> ALTQSVGGDSSADRLFPPQWICCDIRYLDVSILGKFAVVMADPPWDIHMELPYGTLTDDEMRRLNIPVLQDDGFLFLWVTGRAMELGRECLNLWGYERVDEIIWVKTNQLQRIIRTGRTGHWLNHGKEHCLVGVKGNPQGFNQGLDCDVIVAEVRSTSHKPDEIYGMIERLSPGTRKIELFGRPHNVQPNWITLGNQLDGIHLLDPDVVARFKQRYPDGIISKPKNL;> LKGTQSLNPHNDYCQHFVDTGHRPQNFIRDVGLADRFEEYPKLRELIRLKDELIAKSNTPPMYLQADIEAFDIRELTPKFDVILLEPPLEEYYRETGITANEKCWTWDDIMKLEIDEIAAPRSFIFLWCGSGEGLDLGRVCLRKWGYRRCEDICWIKTNKNNPGKTKTLDPKAVFQRTKEHCLMGIKGTVKRSTDGDFIHANVDIDLIITEEPEIGNIEKPVEIFHIIEHFCLGRRRLHLFGRDSTIRPGWLTVGPTLTNSNYNAETYASYFSAPNSYLTGCTEEIERL

The m6A RNA modification is catalyzed in the nucleus by a multiprotein writer complex containing the putative methyltransferases METTL3 and METTL14. The m6A writer complex catalyzes the transfer of a methyl group from the donor substrate S-adenosyl methionine (SAM) to the adenine nucleobases in acceptor RNA substrates. Crucially, our structural and biochemical data imply that METTL3 is the sole catalytic subunit of the complex, while METTL14 plays non-catalytic roles in complex stabilization and substrate RNA recruitment. The structures of the METTL3-METTL14 complex reveal that the two methyltransferase subunits form a compact pseudosymmetric heterodimer with overall dimensions of 80 × 40 × 35 Å.

The truncated METTL3-METTL14 complex was crystallized and its structure solved by a single-wavelength anomalous diffraction approach utilizing the anomalous signal of native sulfur atoms. Experimentally-phased electron density maps revealed the presence of a single molecule of the donor product S-adenosyl homocysteine (SAH), serendipitously co-purified with the complex, in the METTL3 active site. High-resolution native data were subsequently measured from a METTL3-METTL14 crystal grown in the presence of SAH and a short m6A-containing oligonucleotide. However, the RNA oligonucleotide was not evident in electron density maps. The final atomic model, containing a single METTL3-METTL14 dimer in the asymmetric unit, was refined at a resolution of 1.85 Å with an Rfree of 19.0%, working R of 15.7%, and good stereochemistry. Comparisons with the structure of the SAH product-bound complex reveal that the both SAM and SAH molecules adopt very similar conformations except for a slight rotation of the ribose moiety in SAH. Additional ordering of ASL1 is observed in the SAH-bound structure, whereby Tyr406METTL3 caps the SAH product and makes a hydrogen bonding interaction with Ser511METTL3 in ASL2. No additional electron density attributable to SAM or SAH could be observed in the proximity of METTL14 in the two structures. Disulfide bridge formation was observed between Cys338METTL14 and Cys388METTL14.>GAEIPKEMLRAQTNYILRWVLKQGDNYVYGIIKQVKEASNGEMELNEATLYTIFKRLEKDGIISSYWGDESQGGRRKYYRLTEIGHENNRLYFESWSRVDKIIENLEANKKSEAIKSRGGSGGWSHPQFEK[2x]

In previous work, we have introduced pAF into lactococcal multidrug resistance regulator (LmrR), a small homodimeric protein harbouring a pore that exhibits promiscuous substrate binding capabilities, either by direct incorporation using the dedicated orthogonal translation system (OTS),19 or, preferably, by introduction of p-azidophenylalanine (pAzF), followed by a post-translational Staudinger reduction. Incorporation of aY into protein scaffold LmrR gave rise to an artificial Friedel–Crafts (FC) alkylase exhibiting complementary enantioselectivity to a previous FC-alkylase design using p-aminophenylalanine as catalytic residue in the same protein. X-ray crystal structures of the parent and evolved designer enzymes suggest that the introduced mutations cause a narrowing of the active site and a reorientation of the catalytic –NH2 group. Position V15 resides inside the pore of LmrR, and is the same position of ncAA incorporation as used in earlier works featuring pAF as catalytic residue.

In a following round of evolution, SSM libraries of two additional positions in the neighbourhood of the ncAA, i.e. M8 and N19, were prepared using V15aY_RNY as template (S8†). Several variants from both SSM libraries performed better than the parent, of which mutant V15aY_RNY_N19W (RNYW) showed the largest improvements, giving 98% yield and 93% ee when used as purified protein (Fig. 1b and Table S1†). Remarkably, while V15aY exhibits the characteristic LmrR structure, forming an open pore at its dimeric interface of similar shape and dimensions as observed in other LmrR structures, the V15aY_RNYW_KK structure appears to be more closed and exhibits a narrowed cavity. Furthermore, a significant difference in the rotameric state of the aY side chain is observed (S11†). In contrast, in the evolved variant it is placed closer to the pore centre, directed more towards the central tryptophans. The narrowing of the dimeric interface in the evolved variant can be directly linked to the RNYW mutations, which enhance side chain packing between the α1 and α4 helices. The enhanced packing is stabilized through a combination of hydrophobic interactions, aromatic stacking, and hydrogen bonds. Notably, L18R forms hydrogen bonds with M89N, N88 and N14 in the evolved variant, which may explain the epistatic effect observed in catalysis when the L18R and M89N mutations were combined. Hence, this suggests that the RN mutations are key to forming the observed narrowed dimeric interfaces that appear to be beneficial in FC-alkylations, while the introduced Y and W residues most likely further fine-tune the structure and the interactions responsible for achieving efficient and enantioselective catalysis. Moreover, the close proximity of D100 to the aY residue suggests a potential interaction between the carboxylic residue and the substrates, similar to what has been proposed for V15pAF_RGN.> MNGVLIPHTPIAVDFWSLRRAGTARLFFLSHMHSDHTVGLSSTWARPLYCSPITAHLLHRHLQVSKQWIQALEVGESHVLPLDEIGQETMTVTLLDANHCPGSVMFLFEGYFGTILYTGDFRYTPSMLKEPALTLGKQIHTLYLDNTNCNPALVLPSRQEAAHQIVQLIRKHPQHNIKIGLYSLGKESLLEQLALEFQTWVVLSPRRLELVQLLGLADVFTVEEKAGRIHAVDHMEICHSNMLRWNQTHPTIAILPTSRKIHSSHPDIHVIPYSDHSSYSELRAFVAALKPCQVVPIVSRRPCGGFQDSLSPRISVPLIPDSVQQYMSS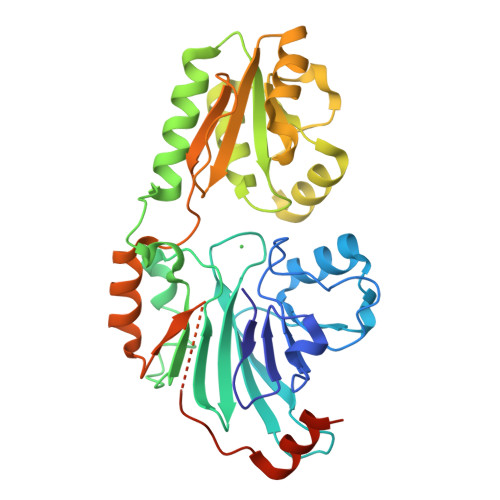SSRKPSAENLYFQ> IVGGYTCAANSIPYQVSLNSGSHFCGGSLINSQWVVSAAHCYKSRIQVRLGEHNIDVLEGNEQFINAAKIITHPNFNGNTLDNDIMLIKLSSPATLDSRVATVSLPRSCAAAGTECLISGWGNTKSSGSSYPSLLQCLKAPVLSDSSCKSSYPGQITGNMICVGFLEGGKDSCQGDSGG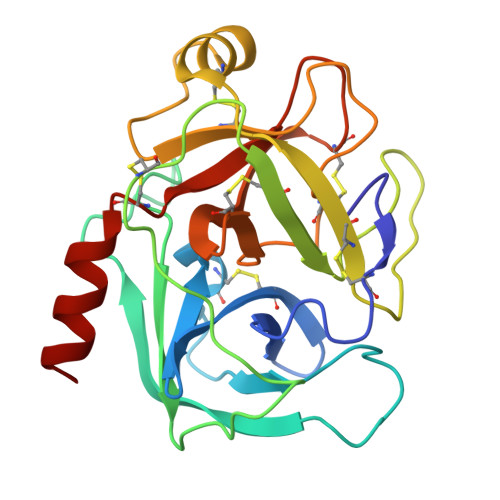PVVCNGQLQGIVSWGYGCAQKNKPGVYTKVCNYVNWIQQTIAAN> MARFNAAFTRIKIMFSRIRGLISCQSNTQTIAPTLSPPSSGHVSFAGIDYPLLPLNHQTPLVFQWFERNPDRFGQNEIPIINT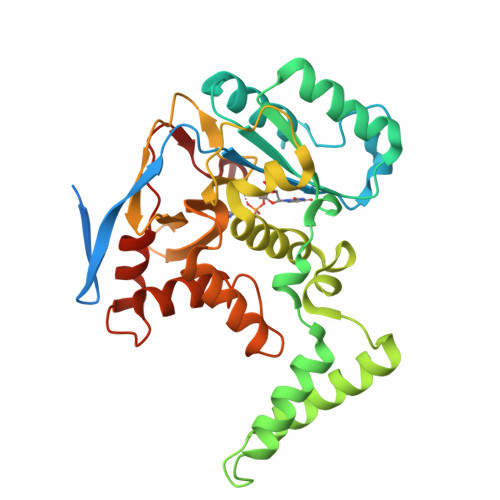QKNPYLNNIINAAIIEKERIIGIFVDGDFSKGQRKALGKLEQNYRNIKVIYNSDLNYSMYDKKLTTIYLENITKLEAQSASERDEVLLNGVKKSLEDVLKNNPEETLISSHNKDKGHLWFDFYRNLFLLKGSDAFLEAGKPGCHHLQPGGGCIYLDADMLLTDKLGTLYLPDGIAIHVSRKDNHVSLENGIIAVNRSEHPALIKGLEIMHSKPYGDPYNDWLSKGLRHYFDGSHIQDYDAFCDFIEFKHENIIMNTSSLTASSWR> MNHLPVVGEDYVEIPDGRPFAPLAGKIEVVEIFGYTCPHCAHFDSKLQAWGARQAKDVRFTLVPAVFGGVWDPFARAYLAADVLGVAKRSHTAMFEA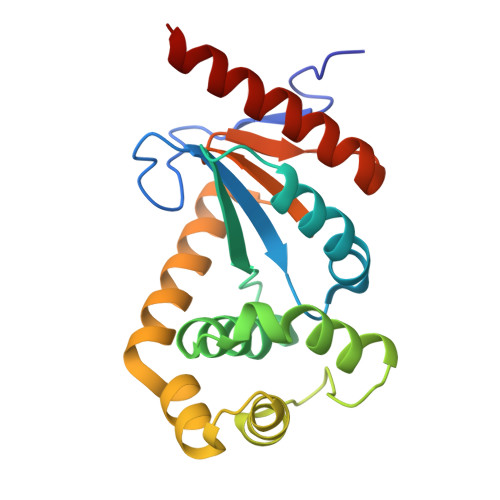IHEKGSVPIQNVGPDELAVFYAGYGVQPDRFVATFNGPEVEKRFQAARAYALKVRPVGTPTIVVNGRYMVTGHDFEDTLRITDYLVSRERAASHGR Proline racemase of Trypanosoma cruzi (TcPRAC) is an enzyme present at all stages of the parasite life cycle, contributing to immune escape and persistence of the parasite in the host. Gene over-expression increases virulence, while knockdown appears lethal for T. cruzi. The structure also showed that TcPRAC crystallizes as a homodimer and bears a catalytic site on each subunit.

Compound 6 (NG-P27), bearing a five-membered ring (reminiscent of proline) was the most active derivative. The NG-P27 compound was co-crystallized with TcPRAC in the same conditions as the BrOxoPA complex. Continuous electron density was observed from residues 38–394 in chain A and 43 to 398 in chain B. Difference Fourier electron density maps indicate the presence of the inhibitor NG-P27 covalently bound to Cys300 in the active site of both polypeptide chains in the dimer. Electron density maps suggested possible multiple conformations of the cyclopentanone moiety of the inhibitor, but no attempt was made to refine alternative conformers and we describe here a single conformation of the ligand that best fits the electron density. The C2 atom of NG-P27 is covalently linked to the sulfur Sγ atom of the catalytic Cys300. In both monomers the inhibitor is very tightly packed, making numerous van der Waals contacts in the active site, and a hydrogen-bonding network stabilizes the carboxylate moiety of NG-P27 as observed for the TcPRAC/BrOxoPA complex. NG-P27, with prochiral substituents on C3, can form a second stereocenter. According to the crystallographic data, the 2S,3R configuration prevailed. Hence, the inhibitor, with C2 positioned si-face adjacent to Cys300, allowed nucleophilic addition (S) through to a mesomeric enolate intermediate. The apparent exponential kinetics constant (kobs) varied linearly with the concentration of OxoPA and NG-P27 as expected for an irreversible inhibition mechanism (inset). These results indicate that NG-P27 is a significantly more potent inhibitor than OxoPA.

>[2x]MGQEKLLFDQKYKIIKGEKKEKKKNQRANRREHQQKREIMRFKKSFTCIDMHTEGEAARIVTSGLPHIPGSNMAEKKAYLQENMDYLRRGIMLEPRGHDDMFGAFLFDPIEEGADLGIVFMDTGGYLNMCGHNSIAAVTAAVETGIVSVPAKATNVPVVLDTPAGLVRGTAHLQSGTESEVSNASIINVPSFLYQQDVVVVLPKPYGEVRVDIAFGGNFFAIVPAEQLGIDISVQNLSRLQEAGELLRTEINRSVKVQHPQLPHINTVDCVEIYGPPTNPEANYKNVVIFGNRQADRSPCGTGTSAKMATLYAKGQLRIGETFVYESILGSLFQGRVLGEERIPGVKVPVTKDAEEGMLVVTAEITGKAFIMGFNTMLFDPTDPFKNGFTLKQYIWSSSVDKLAAALEHHHHHH>TTGSFCPGPVTLCSDLESHSTEAVLGDALVDFSLKLYHAFSAMKKVETNMAFSPFSIASLLTQVLLGAGENTKTNLESILSYPKDFTCVHQALKGFTTKGVTSVSQIFHSPDLAIRDTFVNASRTLYSSSPRVLSNNSDANLELINTWVAKNTNNKISRLLDSLPSDTRLVLLNAIYLSAKWKTTFDPKKTRMEPFHFKNSVIKVPMMNSKKYPVAHFIDQTLKAKVGQLQLSHNLSLVILVPQNLKHRLEDMEQALSPSVFKAIMEKLEMSKFQ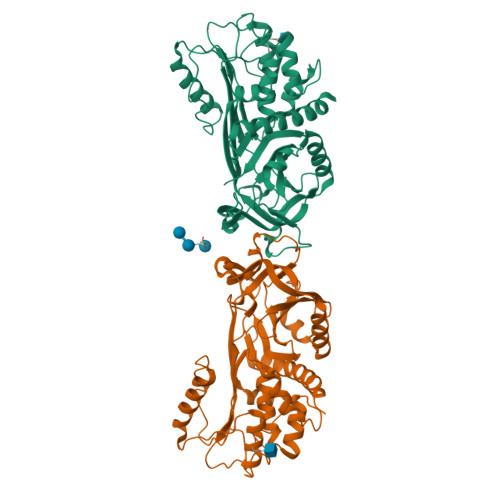PTLLTLPRIKVTTSQDMLSIMEKLEFFDFSYDLNLCGLTEDPDLQVSAMQHQTVLELTETGVEAAAASAISVARTLLVFEVQQPFLFMLWDQQHKFPVFMGRVYDPRA[2x]> IYKTSKEIQKSDQRIIQQRVENSIINNQIYQKSLKRKTSKRKVRHQANKKNFQKEMSEVEDTLNRIKTHKTVLGYLIVNSEGGVVRGAFKDEEESKNIANSIPLLTKKARSVVRDLDPTNDLVFLRIQTK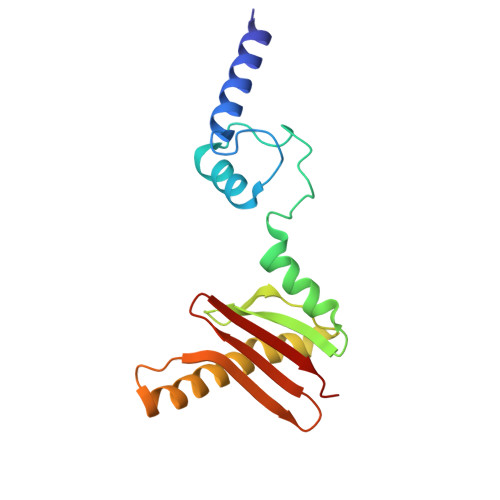LNEIMVAPDDEFSLIVIQTKG> MSTRPRRHAAQRASQAITDLADRDRESDHSHGPISSRMSSFNSSSRSRLPGKGIASVSRSEAGGASDPEHIHLTVKLPSSKLRQATSSSGIKKAGSVGSSSSSSGGGKAAVKRARGGKRSRVLESSEEEEEENEVEVLGDEDEEEEEEEDEIEVREGEGYDEDEEDVEDEDEEMQDLGEEDADGEDDEMDVD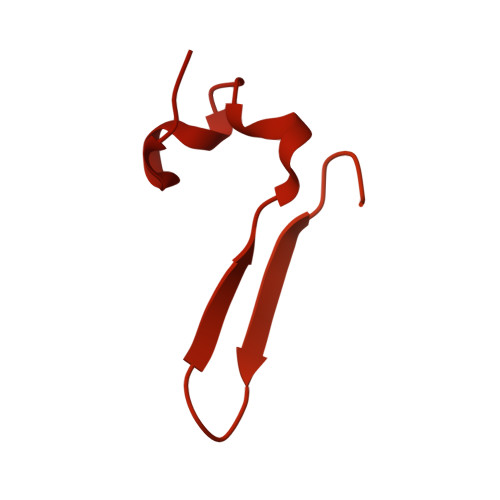AEGEEDADGDVNMDAGVVGARATTVRAVPPAIKVTKPPKESPSNGKAATASKANDNAVPVKRPAPDSDDESLSSLESEPEEEVNVAGGEDAEGEDDDAEGEVDAEGEEEEEEEEIEVADEDAEGEDVEQDEDEDEEEEDDDDEMISRAQTPDMSRLTARQRARLGEASGEYLKLSDEVQSKKHFTAEELSMRRAEMARRRRNLSEKRNEEIKMETVNKLLKKQAPRTTRRAAQAAAAAEEAEEAAKQPKRPDPMMIRWVNNKMGSVVAVPEELLGTHAGVVFGAGPGKGLPAGKMVEEV CSF1R is a type III receptor tyrosine kinase expressed on microglia and macrophages. Colony-stimulating factor 1 receptor (CSF1R) is a key signaling node in microglia and macrophage biology. In particular, CSF1R signaling modulates proliferation, migration, differentiation, and survival of microglia and macrophages in health and disease. Upon CSF1 ligand binding, CSF1R dimerizes and undergoes receptor auto-phosphorylation.

To alter the harmful neuroinflammatory response in progressive MS, we generated a small-molecule CSF1R inhibitor with activity against both mouse and human CSF1R. Specifically, we developed (S)-4-(3-((2-(6-methoxypyridin-3-yl)-2,3-dihydrobenzo[b] dioxin-6-yl)methyl)-3H-imidazo [4,5-b]pyridin-6-yl)-2-methylbut-3-yn-2-amine (sCSF1Rinh) as a result of a structure-based discovery effort aimed at the identification of potent and selective CSF1R inhibitors. sCSF1Rinh, is a type II kinase inhibitor, that binds to CSF1R in a DFG-out conformation. The compound makes a key hydrogen bond interaction to hinge-region residue Cys-666 through N-3 of the imidazo[4,5-b]pyridine ring. The benzodioxane moiety occupies an allosteric pocket adjacent to the ATP binding site, and a second key hydrogen bond interaction is made between O-1 of the benzodioxane ring and Asp-796 of the DFG motif. The alkynylamine function located on the imidazo[4,5-b]pyridine ring extends from the ATP pocket into solvent-exposed space. The binding specificity of sCSF1Rinh was assessed in an active site-directed competition binding assay (KINOMEscan) to measure the interactions between sCSF1Rinh and 450 human kinases and disease-relevant mutant variants. sCSF1Rinh is highly selective for CSF1R as compared to other kinases with a selectivity score of S(35) = 0.005. Furthermore, sCSF1Rinh exhibited excellent pharmacokinetic properties including good oral bioavailability and CNS penetrance, which makes it amenable for both in vitro and in vivo experiments. A short pulse of CSF1 stimulation induced robust CSF1R and ERK1/2 phosphorylation, which was inhibited in the presence of the sCSF1Rinh. We observed similar findings in murine primary microglia and bone marrow-derived macrophages (data not shown) as well as with IL-34 stimulation. Together these data not only show how the kinase activity of CSF1R regulates both its own internalization and degradation, but also demonstrate that sCSF1Rinh effectively inhibits CSF1R signal transduction downstream of the receptor. To interrogate the role of CSF1R in this MS mouse model as well as in macrophage and microglia biology, we developed a novel kinase inhibitor that is potent, selective, and amenable to in vivo experiments.

> YKYKQKPKYQVRWKIIESYEGNSYTFIDPTQLPYNEKWEFPRNNLQFGKTLGAGAFGKVVEATAFGLGKEDAVLKVAVKMLKSTAHADEKEALMSELKIMSHLGQHENIVNLLGACTHGGPVLVITEYCCYGDLLNFLRRKSPPGLEYSYNPSHNPEEQLSSRDLLHFSSQVAQGMAFLASKNCIHRDVAARNVLLTNGHVAKIGDFGLARDIMNDSNYIVKGNARLPVKWMAPESIFDCVYTVQSDVWSYGILLWEIFSLGLNPYPGILVNSKFYKLVKDGYQMAQPAFAPKNIYSIMQACWALEPTHRPTFQQICSFLQEQAQEDRRERD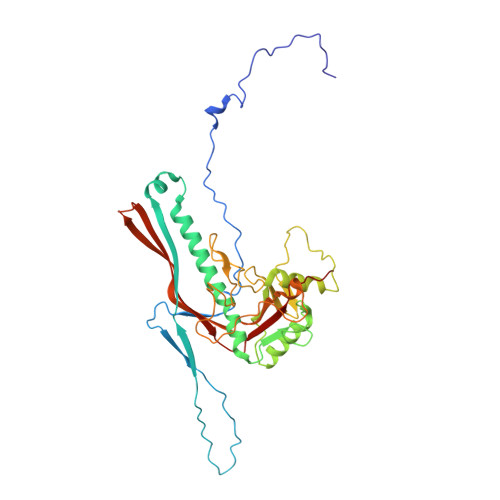> MALNNTTYQGSMRGYAVTKSRLDSFIPEVWTGEVLRALNQNFVASQYVKTLDVTGKKGDRFHIPNIGRASVFDKLPETPVQLQARQESDFYVDIDKYKESSFLIEDLGAMQSSYDIRQEYTTEAGYALSRMMDADILGLRAAVKGLNNGSEIFNTADATISGASSPLNYQALLTAKTILDNRDVPMEKRVIITSPTGYNQLLAIDKFISMDYQDGRPVKSGVVGTIFGIPVIMTTQVTVNSATGYSNGSTVTGIPTPGVSGAGALHLPTQDVFTSLPTAFTGANTGLAAQVITTLMCHSDWAVMLKSKMPSAESDRSVQYLGDIVVNSMVYGAKLFRQTNAVIINHNAVIPAVV> GSASCLELALEGERLCKSGDCRAGVSFFEAAVQVGTEDLKTLSAIYSQLGNAYFYLHDYAKALEYHHHDLTLARTIGDQLGEAKASGNLGNTLKVLGNFDEAIVCCQRHLDISRELNDKVGEARALYNLGNVYHAKGKSFGCPGPQDTGEFPEDVRNALQAAVDLYEENLSLVTALGDRAAQGRAFGNLGNTHYLLGNFRDAVIAHEQRLLIAKEFGDKAAERRAYSNLGNAYIFLGEFETASEYYKKTLLLARQLKDRAVEAQSCYSLGNTYTLLQDYEKAIDYHLKHLAIAQELKDRIGEGRACWSLGNAYT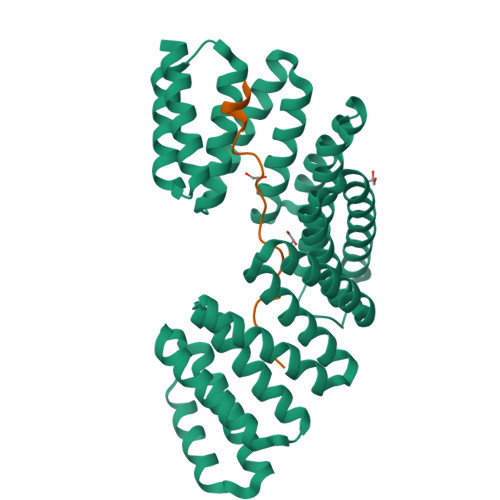ALGNHDQAMHFAEKHLEISREVGD;> RNSFYMGTCQDEPEQLDDWNRIAELQQR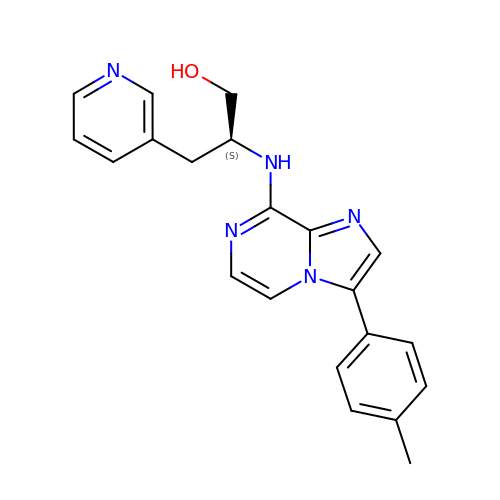(2S)-2-{[3-(4-methylphenyl)imidazo[1,2-a]pyrazin-8-yl]amino}-3-(pyridin-3-yl)propan-1-ol | C21 H21 N5 O | ALAPXRDQVUXCMS-SFHVURJKSA-N> IVGGYTCQENSVPYQVSLNSGYHFCGGSLINDQWVVSAAHCYKSRIQVRLGEHNINVLEGNEQFVNAAKIIKHPNFDHKTLNNDIMLIKLSSPVKLNARVATVALPSSCAPAGTQCLISGWGNTLSSGVNEPDLLQCLDAPLLPQADCEASYPGKITDNMVCVGFLEGGKDSCQGDSGGPVVCNGELQGIV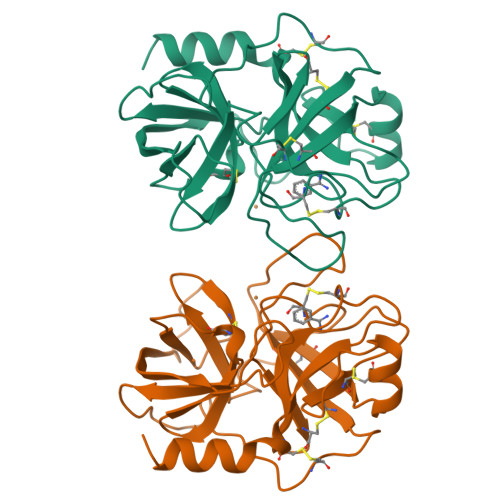SWGYGCALPDNPGVYTKVCNYVDWIQDTIAAN>GSHMEPPPKLVLDLERMAHVPQEKAGPLQRYAATIQSQRGDYNGK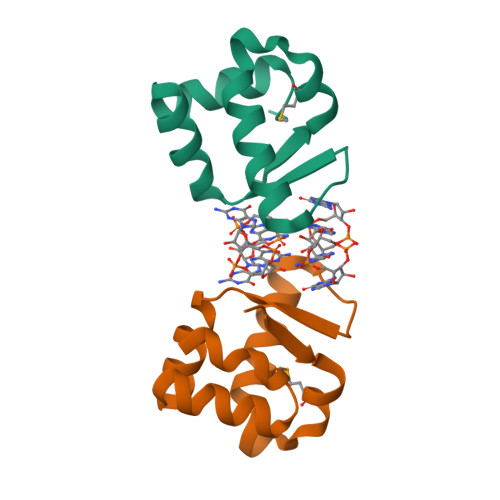VLSIRQDDLRTLAVIYDQSPSVLTEQLISWGVLDADARRAVAHEEN[12x]N-ACETYL-N-[1-(1,1'-BIPHENYL-4-YLMETHYL)-2-OXOAZEPAN-3-YL]-4-[DIFLUORO(PHOSPHONO)METHYL]PHENYLALANINAMIDE | C31 H34 F2 N3 O6 P | 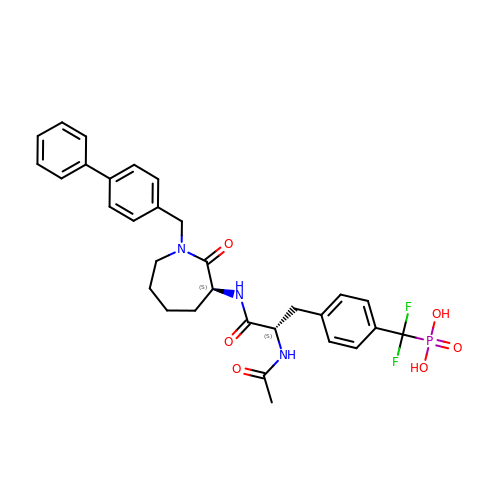LVZDQVATAQEMCX-NSOVKSMOSA-N>MSSAPRRPAKGADSFCTPEPESLGPGTPGFPEQEEDELHRTLGVERFEEILQEAGSRGGEEPGRSYGEEDFEYHRQSSHHIHHPLSTHLPPDARRRKTPQGPGRKPRRRPGASPTGETPTIEEGEEDEDEASEAEGARALTQPSPVSTPSSVQFFLQEDDSADRKAERTSPSSPAPLPHQEATPRASKGAQAGTQVEEAEAEAVAVASGTAGGDDGGASGRPLPKAQPGHRSYNLQERRRIGSMTGAEQALLPRVPTDEIEAQTLATADLDLMKSHRFEDVPGVRRHLVRKNAKGSTQSGREGREPGPTPRARPRAPHKPHEVFVELNELLLDKNQEPQWRETARWIKFEEDVEEETERWGKPHVASLSFRSLLELRRTLAHGAVLLDLDQQTLPGVAHQVVEQMVISDQIKAEDRANVLRALLLKHSHPSDEKDFSFPRNISAGSLGSLLGHHHGQGAESDPHVTEPLMGGVPETRLEVERERELPPPAPPAGITRSKSKHELKLLEKIPENAEATVVLVGCVEFLSRPTMAFVRLREAVELDAVLEVPVPVRFLFLLLGPSSANMDYHEIGRSISTLMSDKQFHEAAYLADEREDLLTAINAFLDCSVVLPPSEVQGEELLRSVAHFQRQMLKKREEQGRLLPTGAGLEPKSAQDKALLQMVEAAGAAEDDPLRR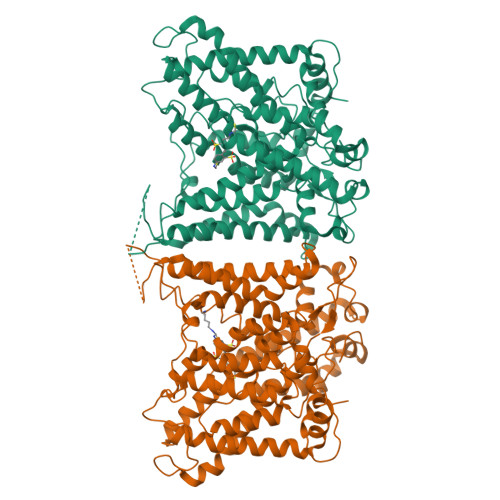TGRPFGGLIRDVRRRYPHYLSDFRDALDPQCLAAVIFIYFAALSPAITFGGLLGEKTQDLIGVSELIMSTALQGVVFCLLGAQPLLVIGFSGPLLVFEEAFFSFCSSNHLEYLVGRVWIGFWLVFLALLMVALEGSFLVRFVSRFTQEIFAFLISLIFIYETFYKLVKIFQEHPLHGCSASNSSEVDGGENMTWAGARPTLGPGNRSLAGQSGQGKPRGQPNTALLSLVLMAGTFFIAFFLRKFKNSRFFPGRIRRVIGDFGVPIAILIMVLVDYSIEDTYTQKLSVPSGFSVTAPEKRGWVINPLGEKSPFPVWMMVASLLPAILVFILIFMETQITTLIISKKERMLQKGSGFHLDLLLIVAMGGICALFGLPWLAAATVRSVTHANALTVMSKAVAPGDKPKIQEVKEQRVTGLLVALLVGLSIVIGDLLRQIPLAVLFGIFLYMGVTSLNGIQFYERLHLLLMPPKHHPDVTYVKKVRTLRMHLFTALQLLCLALLWAVMSTAASLAFPFILILTVPLRMVVLTRIFTDREMKCLDANEAEPVFDEREGVDEYNEMPMPV[2x]Aminoacyl-tRNA synthetases (ARSs) catalyze the ligation of each amino acid to the 3’ hydroxyl group of the cognate tRNA and thereby establish the genetic code for protein synthesis. ARSs assemble into a multi-synthetase complex (MSC), which is comprised of nine ARSs (arginyl- (RARS1), aspartyl- (DARS1), glutaminyl- (QARS1), glutamyl-proryl- (EPRS1), isoleucyl- (IARS1), leucyl- (LARS1), lysyl- (KARS1), and methionyl-tRNA synthetase 1 (MARS1)) and three auxiliary proteins (ARS-interacting multifunctional proteins, AIMP1 (p43), AIMP2 (p38), and AIMP3 (p18)) in vertebrates. IARS1 is one of the least characterized ARSs in the MSC. It is a class 1a ARS and has an UNE-I domain at its C-terminal end that is formed by tandem ~90 residue repeats. The overall structure of GgEARS1 consists of an N-terminal catalytic domain (acceptor end-binding and dinucleotide-binding domains) and C-terminal anticodon-binding domain (proximal β-barrel (Pβ) and distal β-barrel (Dβ) domains).

We also determined the apo GgEARS1 (residues 176–706) structure at 2.5 Å resolution. The helical subdomain (stem-binding domain) connects the catalytic and anticodon-binding domains. The electron density map of both the Pβ and Dβ domains showed significant disorder in the apo GgEARS1 structure, indicating that the regions are highly mobile. However, these regions become ordered upon binding to the IARS1 C-terminal domain, which consists of three repeats of a β-grasp domain. GgEARS1 contains a distinct hairpin loop unique to vertebrate EARS1s in the Pβ domain. This loop is located at the opposite face of the tRNA-binding surface of EARS1 and is oriented perpendicular to the longest axis of GgEARS1. Because the GgEARS1 structure is the first eukaryotic EARS1 structure, we briefly compared it with those of other related ARSs.

> MATEKKADVGKFVELPGAEMGKVIVRFPPEASGYLHIGHAKAALLNQHYQVNFKGKLIMRFDDTNPEKEKEDFEKVILEDVAMLHIKPDQFTYTSDHFETIMKYAEQLIQEGKAYVDDTPAEQMKAEREQRMESKHRNNCVNKNLQMWEEMKKGTEYGQTCCLRAKIDMNSNNGCMRDPTLYRCKNQPHPRTGTTYKVYPTYDFACPIVDSIEGVTHALRTTEYHDRDEQFYWIIEALGIRKPYIWEYSRLNLNNTVLSKRKLMWFVNEGLVDGWDDPRFPTVRGVLRRGMTVEGLKQFIAAQGSSRSVVNMEWDKIWSFNKKVIDPVAPRYTALLKDAVVPVNVPEAQEEMKEVAKHPKNADVGLKPVWYGSKVLIEGADAETLTEGEVVTFINWGNIIITKLNRNSSGKIVSIDTKLNLDNKDFKKTTKITWLAETPRAPLIPTVCVNYEHLITKPVLGKDEDFKQYINRNSKQEELMLGDPCLKDLKKGDIIQLQRRGFFICDQPYEPVSPYSCKEAPCILIYIPDGH4-[(METHYLSULFONYL)AMINO]BENZOIC ACID | C8 H9 N O4 S | 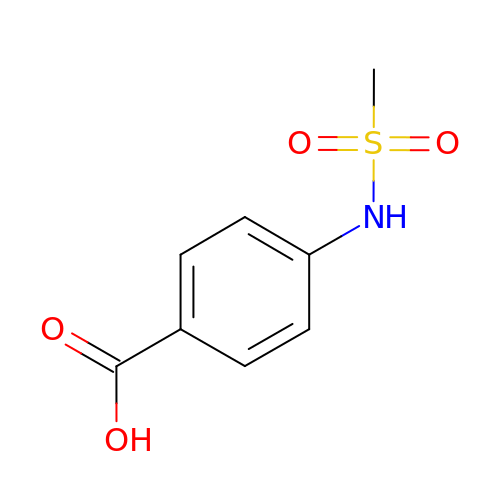SROHFTOYGFCJAF-UHFFFAOYSA-N>[2x]AIKLEHEIKVTDQALFFDGVKKSVPQARTQAYIEGQKYNYAYGNAIAPHGDAIKVYKNYVFMTWYRGGILDRHVMLTRYNTLTGKSVTIEFPHQHTGFEGRWWVGETHNTIAVAISPKDETIHL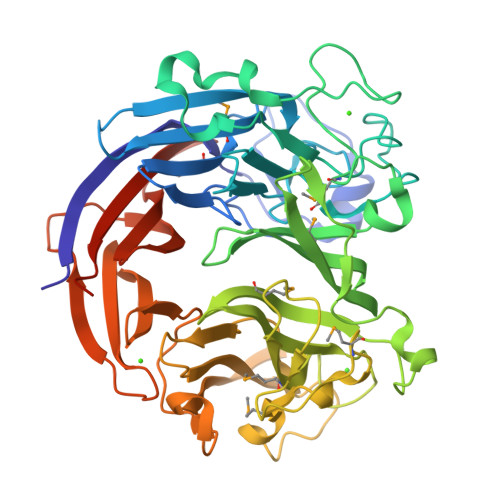LYDMHAYRENTDTGGNGDIRKDYFRYSYSLAGAASVTDNNFTLTQFVKDTSVNSEGATDYKHLTMTGIEDHGQFSRLTYPTFFTSHDGDLFLHMRQGSSHDGRVVFNKYLAEQGKWSHFKSFNVLGAGKKGEIKNWSIYGKMKYADGKIRIGFQRRFNLPDRFRAQDGMFYAYSDDPSGETQWKNYKGEAITMPLVKADEALVMRPGDLLPDATAKDQVSITGGFDWTVTENGDLHLIGQTNEWVNKKVIKKVYSHTYQKAGVGELITTTDFPPASQLYTAGENIYIIGLEQGRPFVEQAKGGTNDFTRVYYAPVGSQSFQKGIVHIHDGKLYYYLLEKGGAGDKRTTYLQIINLDIDSKSYFKKIKQLEHHHHHH> MAEQLKLTKKDRISVWLRSTFLQGSWNYERMQNGGWAYTLIPALKKLYKTKEDRSAALVRHMEFFNTHPYVAAPILGVTLALEEERANGAPIDDVTIQGVKVGMMGPLAGIG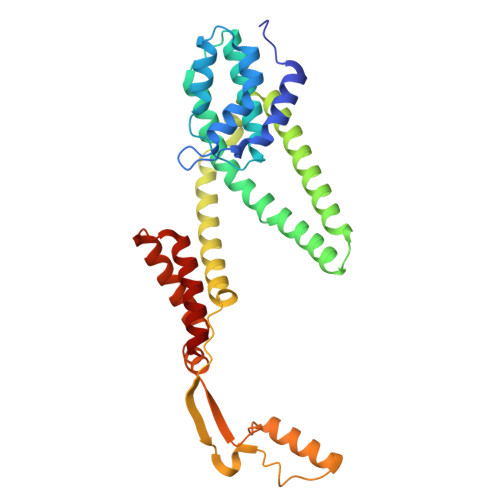DPVFWFTVKPIIGALAASLAMSGNILGPIIYFVAWNAIRMAFTWYTQEFGYRAGSKITEDLSGGILQDITKGASILGMFILGSLVNRWVSVKFTPTVSSVKLDKGAFIDWDKLPSGAKGIQSALQQQAQGLSLTDHKITTLQDNLDSLIPGLAALGLTLFCMWLLKKKVSPIVIILGLFVVGIVFHLLHLM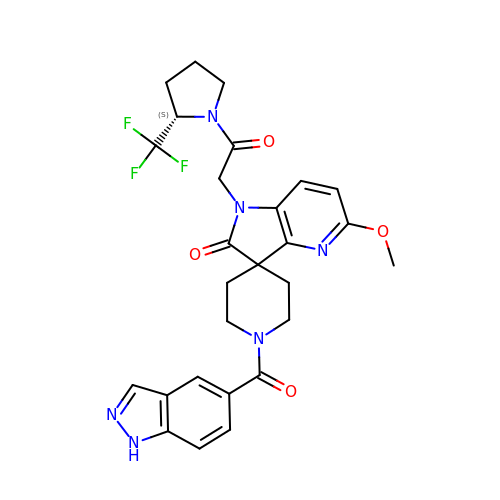1-(1~{H}-indazol-5-ylcarbonyl)-5'-methoxy-1'-[2-oxidanylidene-2-[(2~{S})-2-(trifluoromethyl)pyrrolidin-1-yl]ethyl]spiro[piperidine-4,3'-pyrrolo[3,2-b]pyridine]-2'-one | C27 H27 F3 N6 O4 | ZILKCBIBRQZYMB-FQEVSTJZSA-N>[2x]WQENKSWNAHFTEHKSQGVVVLWNENKQQGFTN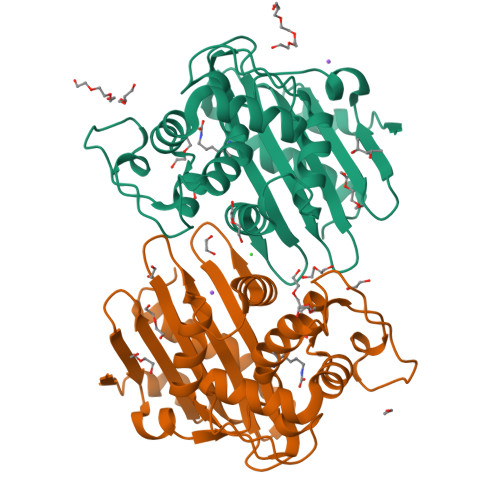NLKRANQAFLPAATFKIPNSLIALDLGVVKDEHQVFKWDGQTRDIATWNRDHNLITAMKYSVVPVYQEFARQIGEARMSKMLHAFDYGNEDISGNVDSFWLDGGIRISATEQISFLRKLYHNKLHVSERSQRIVKQAMLTEANGDYIIRAKTGYSTRIEPKIGWWVGWVELDDNVWFFAMNMDMPTSDGLGLRQAITKEVLKQEKIIP> MKIMMSRRELKEEYKQLEGHPE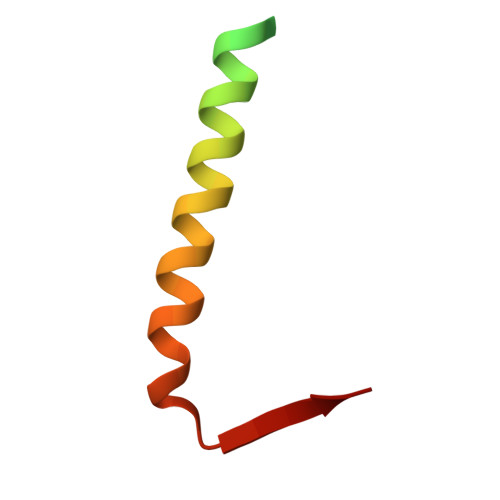VKSRIKARMRELAKSRMMAEVPKATVVITN> MEVKEVVVIVKWSGKEYPVDLTDQDTVEVLRHEIFRKTQVRPERQKLLNLKYKGKTAADNVKISALELKP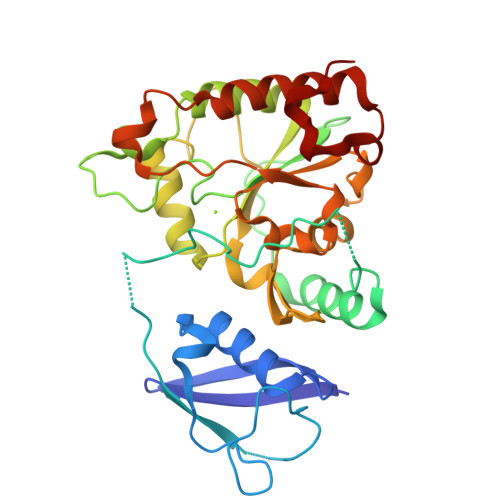NFKLMMVGSTEADIEDACSLPDNIGEVVDDFDDADEREESVAHSAVYLAKVQRRVRDYKIKELAPPREGKKLLVLDIDYTLFDHRSPAETGTELMRPYLHEFLTSAYEDYDIVIWSATSMRWIEEKMRLLGVASNDNYKVMFYLDSTAMISVHVPERGVVDVKPLGVIWALYKQYNSSNTIMFDDIRRNFLMNPKSGLKIRPFRQAHLNRGTDTELLKLSDYLRKIAHHCPDFNSLNHRKWEHYHPKKNS> MSATPAVLRASACSACRFSALRLFVSSFASPRAPLPVARTRVLSPTAPYSTFRPSPRLLASPSSEEHAEPAAQEQPNKTEDAQAEASTEANNEGGADVPWYLQVDAPTHPTLVHEPPPLPDIPEGSPKLMEPLVKFVSDELGMDDLKLLDLREIDPPPALGPEVLMLFGTARSERHLHVSADRLVRWLRNRGVTAKADGLLGRNELKTKLRRKARKAKLLGTTGLPSGADDGITTGWICVNLGTLGWSDMEMEFKDEKGVTSGFGVPQSGTTLVVQLMTETRREELALEKLWSGILRRSLERQDKIAGKLPEASFTTSPDTVSGQSFSPSPIRSSGRNRKRPDRLYFSTSARQHAAAVDVSQTDLATAMA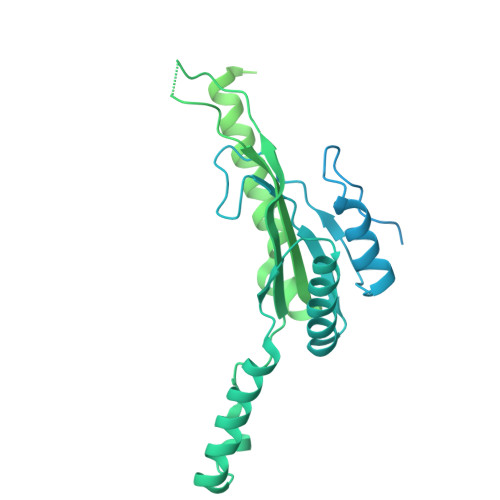GWEYSNASPSTIDNLLAQDTDSKVQLLIQMQEYLSSLPRDQALSAVSLCEDGSPSTFMRLFNRAIENLPSAQAWEARLWVEKAARALQHPDHDLARLGDLIQEMKLSGAANVSREKFVDLLRMIFAIPETTDAGVRQQASLSMDVIDMLFSRGEKVIEYDVVVAVIESLLQTRARPPEARRLLSQFEDLLSEAQMDCPTEDEIIRLLDVYANHRAWDKFWNVWRVFPRHCERRTERMYTKVYERIAAEDHQGMATDALRWCVEEMWHEQPPVRVTAAMLKALEACIRIADPEAESLAKDIDDRISDAQYMDREFVRLWLTLHGSAAWGA>[4x]MKHLHRFFSSDASGGIILIIAAILAMIMANSGATSGWYHDFLETPVQLRVGSLEINKNMLLWINDALMAVFFLLVGLEVKRELMQGSLASLRQAAFPVIAAIGG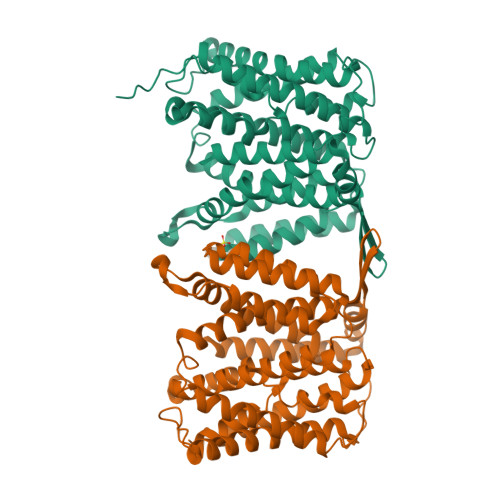MIVPALLYLAFNYADPITREGWAIPAATDIAFALGVLALLGSRVPLALKIFLMALAIIDDLGAIIIIALFYTNDLSMASLGVAAVAIAVLAVLNLCGARRTGVYILVGVVLWTAVLKSGVHATLAGVIVGFFIPLKEKHGRSPAKRLEHVLHPWVAYLILPLFAFANAGVSLQGVTLDGLTSILPLGIIAGLLIGKPLGISLFCWLALRLKLAHLPEGTTYQQIMVVGILCGIGFTMSIFIASLAFGSVDPELINWAKLGILVGSISSAVIGYSWLRVRLRPSVEFRVPGSENLYFQ>[2x]MAPHRPAPALLCALSLALCALSLPVRAATASRGASQAGAPQGRVPEARPNSMVVEHPEFLKAGKEPGLQIWRVEKFDLVPVPTNLYGDFFTGDAYVILKTVQLRNGNLQYDLHYWLGNECSQDESGAAAIFTVQLDDYLNGRAVQHREVQGFESATFLGYFKSGLKYKKGGVASGFKH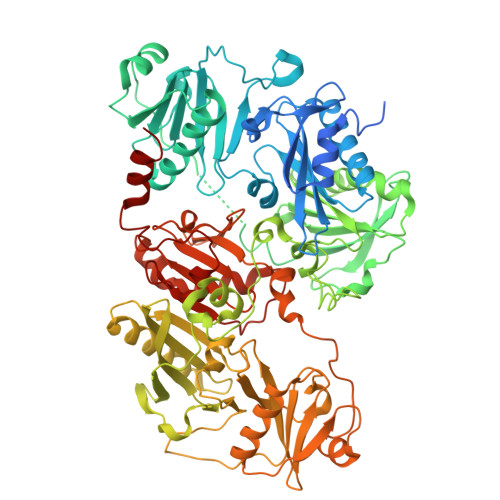VVPNEVVVQRLFQVKGRRVVRATEVPVSWESFNNGDCFILDLGNNIHQWCGSNSNRYERLKATQVSKGIRDNERSGRARVHVSEEGTEPEAMLQVLGPKPALPAGTEDTAKEDAANRKLAKLYKVSNGAGTMSVSLVADENPFAQGALKSEDCFILDHGKDGKIFVWKGKQANTEERKAALKTASDFITKMDYPKQTQVSVLPEGGETPLFKQFFKNWRDPDQTDGLGLSYLSSHIANVERVPFDAATLHTSTAMAAQHGMDDDGTGQKQIWRIEGSNKVPVDPATYGQFYGGDSYIILYNYRHGGRQGQIIYNWQGAQSTQDEVAASAILTAQLDEELGGTPVQSRVVQGKEPAHLMSLFGGKPMIIYKGGTSREGGQTAPASTRLFQVRANSAGATRAVEVLPKAGALNSNDAFVLKTPSAAYLWVGTGASEAEKTGAQELLRVLRAQPVQVAEGSEPDGFWEALGGKAAYRTSPRLKDKKMDAHPPRLFACSNKIGRFVIEEVPGELMQEDLATDDVMLLDTWDQVFVWVGKDSQEEEKTEALTSAKRYIETDPANRDRRTPITVVKQGFEPPSFVGWFLGWDDDYWSVDPLDRAMAELAA>[2x]MHHHHHHSSGRENLYFQGKMWKPGDECFALYWEDNKFYRAEVEALHSSGMTAVVKFIDYGNYEEVLLSNIKPIQTE

Survival of motor neuron (SMN) functions in diverse biological pathways via recognition of symmetric dimethylarginine (Rme2s) on proteins by its Tudor domain, and deficiency of SMN leads to spinal muscular atrophy. Here we report a potent and selective antagonist with a 4-iminopyridine scaffold targeting the Tudor domain of SMN. In order to understand the structural basis of compound 1 recognition by these reader proteins, we determined the crystal structures of compound 1 in complex with SMN, TDRD3 and UHRF1, respectively. In this study, we identified some low micromolar antagonists with a 4-iminopyridine scaffold targeting the Tudor domain of SMN, and compound 1 shows >4-fold selectivity over other tested methyllysine or methylarginine binding domains.

SMN, SMNDC1 and TDRD3 are the only three known methylarginine binding proteins of single canonical Tudor domain. UHRF1_TTD was the only assayed methyllysine binder that bound to compound 1 measurably, and compound 1 bound more tightly to the methylarginine binding Tudor domains of SMN, SMNDC1, and TDRD3 than to the methyllysine binding Tudor domain of UHRF1_TTD. Moreover, the highly homologous Tudor domains of SMN and SMNDC1 bound to compound 1 with a ~4-fold selectivity over that of TDRD3. In the TDRD3-compound 1 structure, the binding mode is largely conserved, but Y566 of TDRD3 might not stack with the compound as effectively as W102 in SMN, which may explain weaker binding affinity of TDRD3 to compound 1. Consistent with this hypothesis, the W102Y mutant of SMN showed a binding affinity to compound 1 similar to wild-type TDRD3, and the Y566W mutant of TDRD3 displayed a binding affinity to compound 1 similar to wild-type SMN.In the present study, the gene product of gene ID 9704440, here referred to as MmNQO, was cloned, overexpressed in E. coli and characterized biochemically and structurally. Based on the results from these analyses, gene ID 9704440 codes for a soluble protein of 196 amino acids. Based on structural and biochemical data, we suggest that FMN and NADH are preferred, which justifies that MmNQO is annotated as an FMN-dependent NADH:quinone oxidoreductase. The biological function of MmNQO is yet to be elucidated, but from the data presented here it may constitute an archaeal counterpart of the modulator of drug activity B in bacteria.

The crystal structure of MmNQO features a homodimeric enzyme where each monomer adopts the flavodoxin-like α/β-fold commonly observed for NAD(P)H:quinone oxidoreductases. The active sites of both monomers are situated at the dimer interface, each with a non-covalently bound FMN molecule bound approximately 8 Å below the molecule's surface. The flavin isoalloxazine ring is firmly bound by the protein with its dimethylbenzene nucleus interacting with hydrophobic side chains (Trp89and Trp90 from molecule A; and Leu48 and Tyr53 from molecule B); the N5 atom of the central phenylenediamine ring forming a hydrogen bond to the backbone amide nitrogen of Trp90; and the O2 and O4 oxygen atoms in the pyrimidine of the isoalloxazine ring forming hydrogen bonds to the backbone amide groups of His135 and Ser91, respectively. There are two non-crystallographically related homodimers (A/B and C/D) in the asymmetric unit of the crystal. In each dimer, one monomer (A in the A/B dimer and C in the C/D dimer) packs such that the ultimate histidine of the C-terminal hexahistidine tag is reaching into the flavin pocket to interact with the FMN ring in a crystallographically related molecule, i.e. His203 in molecule A interacts with the FMN in a crystallographically related D monomer and Asp156 in a crystallographically related C monomer. This interaction places the A-His203 CE1 atom 3.1 Å from the O4 atom of D-FMN. Although local conformational changes may well change the precise details and relieve steric hindrance, His135 is very strategically positioned at one side of the FMN cofactor to restrict the substrate-binding region, a feature that does not exist in bacterial FMN azoreductases. At the sequence level, the region responsible for binding the adenosine part of FAD in SmMdaB is overall very similar in MmNQO, i.e. loop A (residues 9–15) and loop F (residues 173–182), including an important interaction offered by His9 to the FMN α-phosphate group. An additional interaction to the monophosphate is provided by Tyr53 in MmNQO, which is absent in SmMdaB. In the FMN-bound state of MmNQO, loop F is folded around the monophosphate moiety whereas in the FAD-bound state of SmMdaB, the F-loop is folded away to accommodate the adenosine ring.

>[4x]MASMHVYILFAHPSRKSFSREVLEAFTEGLSEAGHTYEVGDLYRMNFRSELSQEEYLREISQEAGSPLPEDVMEEHERIGRADALAFIYPLWWSDCPAKLKGWFDRVWTYGYAYFYEDGERGTRIDIEKAVVLCSAGHTEEDLEGTGIAESMRSVMLGDRLLGVGVKNVTMEILGGMVPGDDSCREINLMRARRAGRNLEHHHHHH>MHESVTANIENV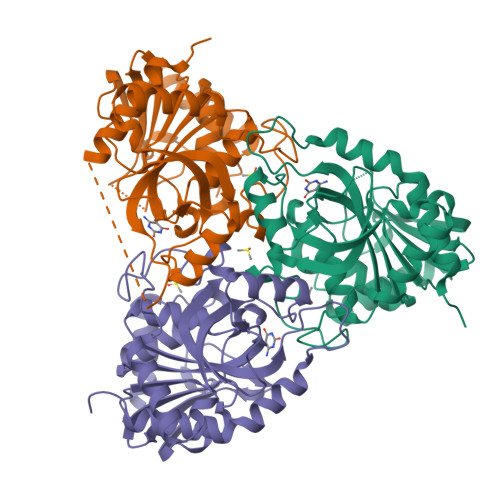KKVAHHIQKLTSIVPEIGIICGSGLGKLADGVKDKITIPYTKIPNFPQTSVVGHSGNLIFGTLSGRKVVVMQGRFHMYEGYSNDTVALPIRVMKLLGVKILMVSNAAGGLNRSLKLGDFVILKDHIYLPGLGLNNILVGPNQEAFGTRFPALSNAYDRDLRKLAVQVAEENGFGNLVHQGVYVMNGGPCYETPAECTMLLNMGCDVVGMSTIPEVVIARHCGIQVFAVSLVTNISVLDVESDLKPNHEEVLATGAQRAELMQSWFEKIIEKLPKD[3x]>[4x]MTDTP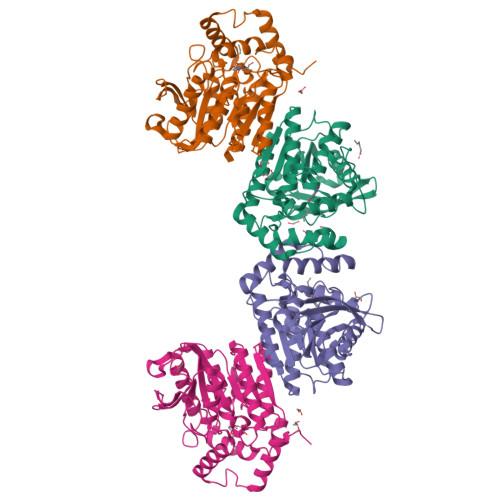FIRPDMKAFLEAIAAMAGPTLAEMTLEEARASYVALHGMADRPARELAVIRNLSCPGPAGDIPLRLYDARESREAGPVITFYHGGGFVIGDLDTHHNLCTEIAALMDLPVVAVDYRLAPEHPFPAAIEDCEAATRWVASSPSELGRTASGVIPIGDSAGGNATIVVSQLLGAKPADVPVVLQVPIFPLASDAVGSASLEAFAEGFVLTKASIEFFDTAYKADRADPRGFPILGDHTAAPPTIVATASLDPLRDSGRDYAKALVEAGRDVVYLEMEGVTHSFTNIRAAVPSTQGDLERIIAAMKMMLGTA>[4x]SPLAAYEVDDSTGYLTSDVGGPIQDQTSLKAGIRGPTLLEDFMFRQKIQHFDHERVPERAVHARGAGAHGTFTSYADWSNITAASFLNATGKQTPVFVRFSTVAGSRGSADTARDVHGFATRFYTDEGNFDIVGNNIPVFFIQDAIQFPDLIHSVKPRPDNEIPQAAFAHDSAWDFFSQQPSTMHTLFWAMSGHGIPRSYRHMDGFGVHTFRFVKDDGSSKLIKWHFKSRQGKASLVWEEAQVLSGKNADFHRQDLWDAIESGNGPEWDVCVQIVDESQAQAFGFDLLDPTKIIPEEYAPLTKLGLLKLDRNPTNYFAETEQVMFQPGHIVRGIDFTEDPLLQGRLFSYLDTQLNRNGGPNFEQLPINMPRVPIHNNNRDGAGQMFIHRNKYPYTPNTLNSGYPRQANQNAGRGFFTAPGRTASGALVREVSPTFNDHWSQPRLFFNSLTPVEQQFLVNAMRFEISLVKSEEVKKNVLTQLNRVSHDVAVRVAAAIGLGAPDADDTYYHNNKTAGVSIVGSGPLPTIKTLRVGILATTSESSALDQAAQLRTRLEKDGLVVTVVAETLREGVDQTYSTADATGFDGVVVVDGAAALFASTASSPLFPTGRPLQIFVDAYRWGKPVGVCGGKSSEVLDAADVPEDGDGVYSEESVDMFVEEFEKGLATFRFTDRFALDS

Catalase (CATPO) from the thermophilic fungus S. thermophilum is a clade 2 enzyme consisting of four subunits, each with a molecular weight of 80 kDa. In addition to its primary catalase activity, it also has a minor phenol oxidase activity that is capable of oxidizing o-diphenolic and some p-diphenolic compounds in the absence of hydrogen peroxide. In large-subunit catalases the gate and small cavity are formed by Arg134, Glu484 (CATPO numbering) and a loop of four residues (Gln185, Ala186, Ala187 and Thr188 in CATPO). The highly conserved four-residue loop located directly above the hydrophobic lower part of the main channel in large-subunit catalases is thought to act as a gate allowing access of H2O2 to the lower part of the main channel, while reducing water access.

The E484A and T188F variants were selected because they have a lower catalase k cat but a higher phenol oxidase activity than CATPO. The E484A and T188F variants showed a decrease in turnover by 53% and 48%, respectively. However, the turnover numbers increased for the E484A (sixfold), E484I (fourfold), T188D (threefold), T188F (fourfold) and T188I (fourfold) variants, while they did not change significantly for the E484D and T188A variants. The presence of heme d in the T188A variant and of heme b in the E484A and T188F variants was also confirmed by crystallographic analysis. Although the K m value did not change compared with the wild-type CATPO enzyme, this mutation had a negative effect on the catalytic activity. In the T188F mutant the solvent distribution in the upper part of the main channel is very different as the phenylalanine protrudes into the channel, while the lower part of the channel is similar to that of wild-type CATPO. The channel appears to be closed in the E484A and T188F variants, which would prevent H2O2 molecules from entering the cavity. This is due to a shift in the position of Thr188 (in the E484A variant) into the channel and the corresponding Phe188 residue in the T188F variant protruding deeply into the channel.> HHHHHHLANTSAHDFSYLKFVYNATDTSLEGSYDYIVIGGGTSGCPLAATLSEKYKVLLLERGTIATEYPNTLTADGFAYNLQQQDDGKTPVERFVSEDGIDNVRARILGGTTIINAGVYARANISFYSQTGIEWDLDLVNKTYEWVEDAIVVKPNNQSWQSVIGEGFLEAGILPDNGFSLDHEAGTRLTGSTFDNNGTRHAADELLNKGDPNNLLVAVQASVEKILFSSNTSNLSAIGVIYTDSDGNSHQAFVRGNGEVIVSAGTIGTPQLLLLSGVGPESYLSSLNITVVQPNPYVGQFVYDNPRNFINILPPNPIEASVVTVLGIRSDYYQVSLSSLPFSTPPFSLFPTTSYPLPNSTFAHIVSQVPGPLSHGSVTLNSSSDVRIAPNIKFNYYSNSTDLANCVSGMKKLGDLLRTKALEPYKARDVLGIDGFNYLGVPLPENQTDDASFETFCLDNVASYWHYHGGSLVGKVLDDSFRVMGIKALRVVDASTFPYEPNSHPQGFYLMLGRYVGLQILQERS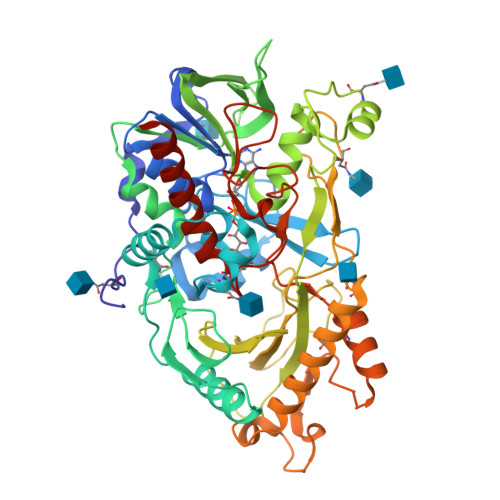IRLEAIHNIQESM>[4x]MIPARFAGVLLALALILPGTLCAEGTRGRSSTARCSLFGSDFVNTFDGSMYSFAGYCSYLLAGGCQKRSFSIIGDFQNGKRVSLSVYLGEFFDIHLFVNGTVTQGDQRVSMPYASKGLYLETEAGYYKLSGEAYGFVARIDGSGNFQVLLSDRYFNKTCGLCGNFNIFAEDDFMTQEGTLTSDPYDFANSWALSSGEQWCERASPPSSSCNISSGEMQKGLWEQCQLLKSTSVFARCHPLVDPEPFVALCEKTLCECAGGLECACPALLEYARTCAQEGMVLYGWTDHSACSPVCPAGMEYRQCVSPCARTCQSLHINEMCQERCVDGCSCPEGQLLDEGLCVESTECPCVHSGKRYPPGTSLSRDCNTCICRNSQWICSNEECPGECLVTGQSHFKSFDNRYFTFSGICQYLLARDCQDHSFSIVIETVQCADDRDAVCTRSVTVRLPGLHNSLVKLKHGAGVAMDGQDVQLPLLKGDLRIQHTVTASVRLSYGEDLQMDWDGRGRLLVKLSPVYAGKTCGLCGNYNGNQGDDFLTPSGLAEPRVEDFGNAWKLHGDCQDLQKQHSDPCALNPRMTRFSEEACAVLTSPTFEACHRAVSPLPYLRNCRYDVCSCSDGRECLCGALASYAAACAGRGVRVAWREPGRCELNCPKGQVYLQCGTPCNLTCRSLSYPDEECNEACLEGCFCPPGLYMDERGDCVPKAQCPCYYDGEIFQPEDIFSDHHTMCYCEDGFMHCTMSGVPGSLLPDAVLSSPLSHRSKRSLSCRPPMVKLVCPADNLRAEGLECTKTCQNYDLECMSMGCVSGCLCPPGMVRHENRCVALERCPCFHQGKEYAPGETVKIGCNTCVCRDRKWNCTDHVCDATCSTIGMAHYLTFDGLKYLFPGECQYVLVQDYCGSNPGTFRILVGNKGCSHPSVKCKKRVTILVEGGEIELFDGEVNVKRPMKDETHFEVVESGRYIILLLGKALSVVWDRH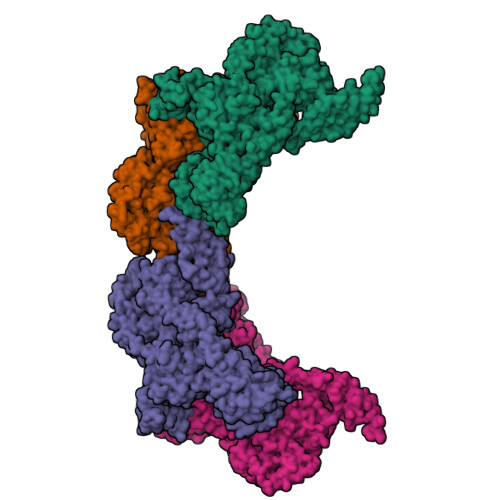LSISVVLKQTYQEKVCGLCGNFDGIQNNDLTSSNLQVEEDPVDFGNSWKVSSQCADTRKVPLDSSPATCHNNIMKQTMVDSSCRILTSDVFQDCNKLVDPEPYLDVCIYDTCSCESIGDCACFCDTIAAYAHVCAQHGKVVTWRTATLCPQSCEERNLRENGYECEWRYNSCAPACQVTCQHPEPLACPVQCVEGCHAHCPPGKILDELLQTCVDPEDCPVCEVAGRRFASGKKVTLNPSDPEHCQICHCDVVNLTCEACQEPG>[4x]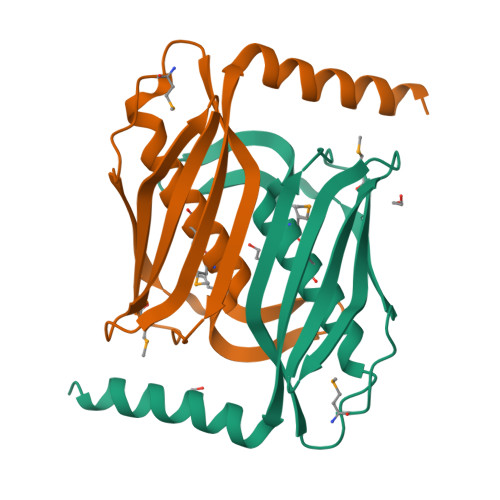MRPIPEGYEAVFETVVTPEMTVRFEELGPVHPVYATYWMVKHMELAGRKIILPFLEEGEEGIGSYVEARHLASALPGMRVRVVARHEKTEGNRVYARVEAYNELGDLIGVGRTEQVILPKAKVEALFRRLKERWEAERSPS>[2x]MTVQCKPIPALYTVYVLRSTVRHASLYIGSTPNPPRRLKQHNGLVPGGAARTSRSSLRPWEMVALVSGFPSMVAALKFQWALTNPHLSVHIPSASRLTVATQTKANGRPQRPPRSLASVVANLHLLLRVPSFARWPLRVHFFRRDVFAAWEKWCAAASERLRPSLAVVTDFEGGSEGLAGAVVGGEEGRERGEGAPCWGIHALPLDYEPIKDYVAKGQEIFEFERQGACVVCREEMASGDGLQALCTNQGCDGVGHLSCWSRHFLKGAEADSILPVQGQCPKCGGEMEWGNMMKELTLRTRGQKEVEKLLKRKRRRATKKTANA;>MEDTETSLVASPTDQQVSLFRYITQAVVTAPRAKDPANPSWHEKMLMYDPIILEDLTAWLNSGQLDRVGYDGEVAPGDVKKWCESKSVCCLWRVSLNGKERKRF[2x]

SLX1 belongs to the GIY-YIG superfamily of nucleases. When bound to SLX4, SLX1 cleaves various branched DNA substrates near the branch point. Slx1 comprises two distinct domains: N-terminal GIY-YIG nuclease domain and C-terminal RING domain which binds two zinc ions. The CCD3 fragment of Slx4 bound between these two domains.

We obtained two crystal forms of Slx1–Slx4CCD3 from Thielavia terrestris (Tt-Slx1–Slx4CCD3, where CCD3 corresponds to a previously characterized Candida glabrata construct). Crystals of Tt-Slx1–Slx4CCD3 that were obtained in the presence of HJs were found to be crystals of protein alone. These apo crystals crystallized in the C 2 space group and diffracted X-rays to a resolution of 3.1 Å. The phases were determined using single-wavelength anomalous diffraction (SAD) for zinc ions at a wavelength of 1.2828 Å. The asymmetric unit contained two molecules. The overall structure of Tt-Slx1–Slx4CCD3 was very similar to Slx1–Slx4CCD3 from Candida glabrata, which was reported earlier. The main difference between them was the connection between the GIY-YIG and RING domains. This region formed a long α-helix in Cg-Slx1–Slx4CCD3, whereas it lacked a secondary structure and was partly disordered in Tt-Slx1–Slx4CCD3. In the apo structure, the region that comprised residues 88–113 was not visible in the electron density maps and was likely disordered.> MVAASMNILSKISSFIGKTFSLWAALFAAAAFFAPDTFKWAGPYIPWLLGIIMFGMGLTLKPSDFDILFKHPKVVIIGVIAQFAIMPATAWCLSKLLNLPAEIAVGVILVGCCPGGTASNVMTYLARGNVALSVAVTSVSTLTSPLLTPAIFLMLAGEMLEIQAAGMLMSIVKMVLLPIVLGLIVHKVLGSKTEKLTDALPLVSVAAIVLIIGAVVGASKGKIMESGLLIFAVVVLHNGIGYLLGFFAAKWTGLPYDAQKALTIEVGMQNSGLAAALAAAHFAAAPVVAVPGALFSVWHNISGSLLATYWAAKAGKHKKPLDRAGS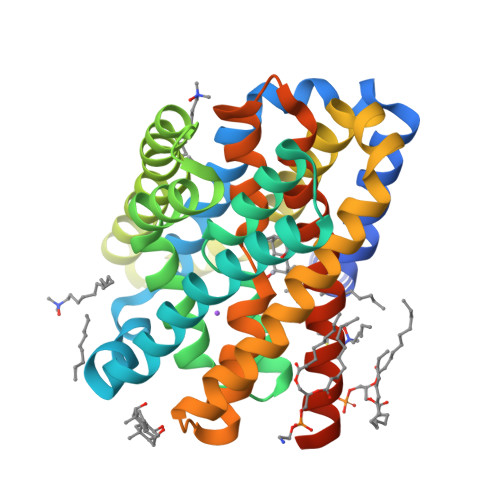ENLYFQ Obtusifoliol | C30 H50 O | 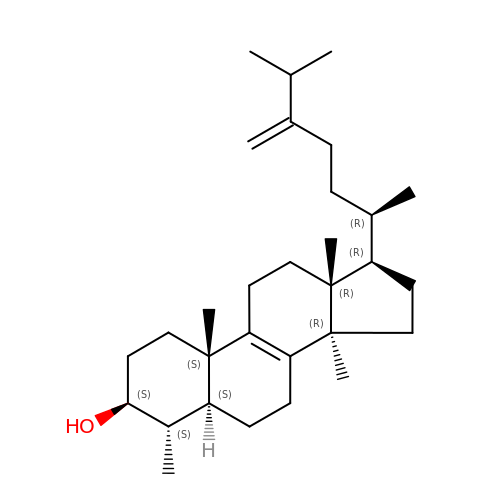MMNYKQIDRZNIKT-VSADUBDNSA-N>MHHHHHHMVGFGELKEEWRGEVVHLSWSPRAFLLKNFLSDEECDYIVEKARPKMVKSSVVDNESGKSVDSEIRTSTGTWFAKGEDSVISKIEKRVAQVTMIPLENHEGLQVLHYHDGQKYEPHYDYFHDPVNAGPEHGGQRVVTMLMYLTTVEEGGETVLPNAEQKVTGDGWSECAKRGLAVKPIKG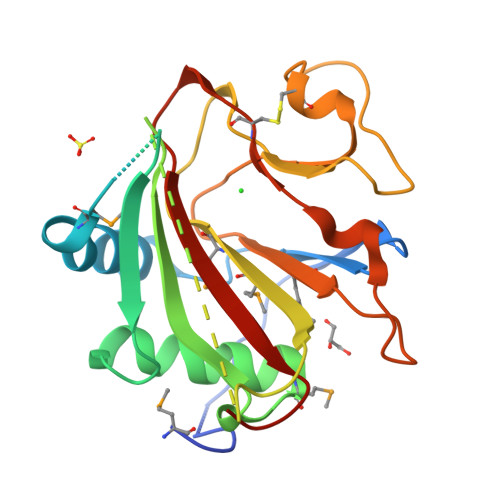DALMFYSLKPDGSNDPASLHGSCPTLKGDKWSATKWIHVAPIGGRH[4x]> MANKVIQLQKIFQSSTKPLWWR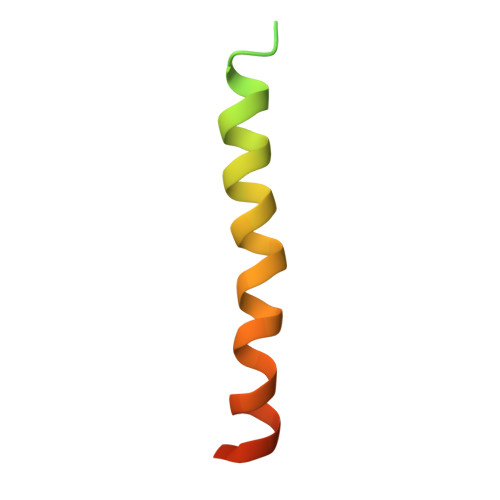HPRSALYLYPFYAIFAVAVVTPLLYIPNAIRGIKAKKA> MSLAKVWTYASWIPRGIPKAMANELSSAAAALAHPEAIARVAQLESQGKNPYRVARAEFWQMYLACWPYRFRNTVVEWETCKAKVLKGSVDLQDIVDLLYLLAWAYLFWILGEIYGRGSLYGYRFDGEIHRQEAQNVILYKEKEAQEMAVVMEKLEKEI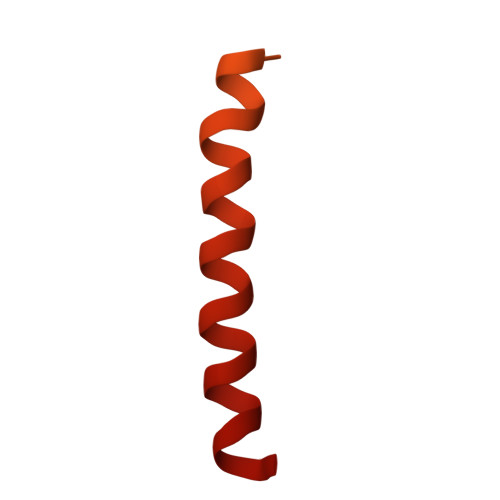QEWLKTMEQE> MNEAVIEKLLENSRKFLTGAKLICQESNDHLTTTKLRIREWQKFQSKLHFVLDCIQQQTKFLSEILLREGIGRNLIEEEWSQTVLVRLVNDMKFWQNEITKMMNKLDNITNEIDQQHNSKLGDFISRDSSHILDSKLNEIPTIRKQVENITRQYQTMLAKVQSQLVESR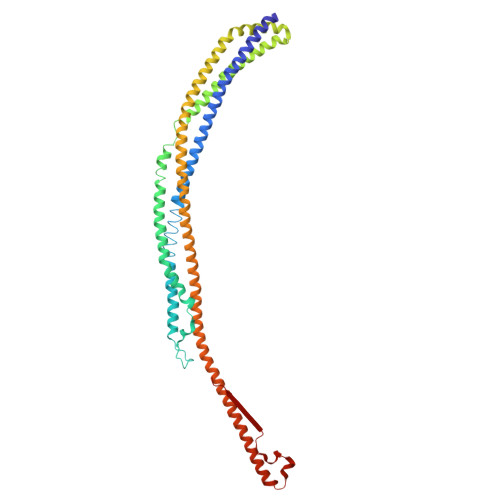MKGLRDEFSSKFGDQCRENLKLNEEFTNEADQLEQELADFLKSFTDHFDKCSALSSRSVSPEDAQNLFEIVERDDKDLAAINSLLQDAAIDVASFVRKVNMLLDERDADKAKMQATLSKLLTELRKHEEYISVFEGISALIQKFKASCLEDIRQTRNLLDFYANFERSYHNLLKEVKRRKETAAKLSQILKSCETQLEQINTADLRERQMFLLENGNYLPETIWPDEIGSLSPLYTLNYEVRKV> RKIKVPENIEEIAREVGQIAKEMGLRAYIVGGVVRDILLGKEVWDVDFVVEGNAIELAKELARRHGVNVHPFPEFGTAHLKIGKLKLEFATARRETYPRPGAYPKVEPASLKEDLIRRDF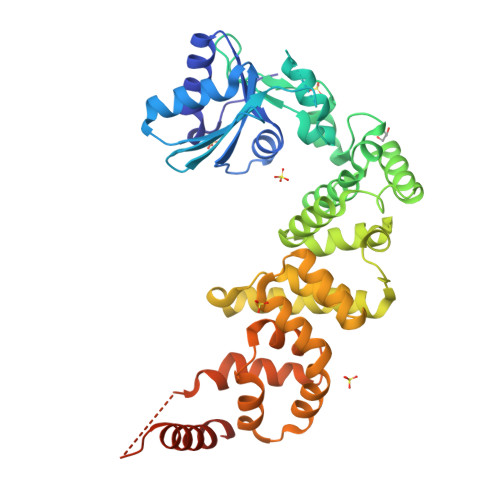TINAMAISVNLEDYGTLIDYFGGLRDLKDKVIRVLHPVSFIEDPVRILRALRFAGRLNFKLSRSTEKLLKQAVNLGLLKEAPRGRLINEIKLALREDRFLEILELYRKYRVLEEIIEGFQWNEKVLQKLYALRKVVDWHALEFSEERIDYGWLYLLILISNLDYERGKHFLEEMSAPSWVRETYKFMKFKLGSLKEELKKAKENYEVYRLLKPLHTSVLLLLMLEEELKEKIKLYLEKLRKVKLPKEKIEELKKQGLKGKELGERIEELKREIMNKIKLAAALEHHHHHH> MRVKTIMTQNPVTITLPATRNYALELFKKYKVRSF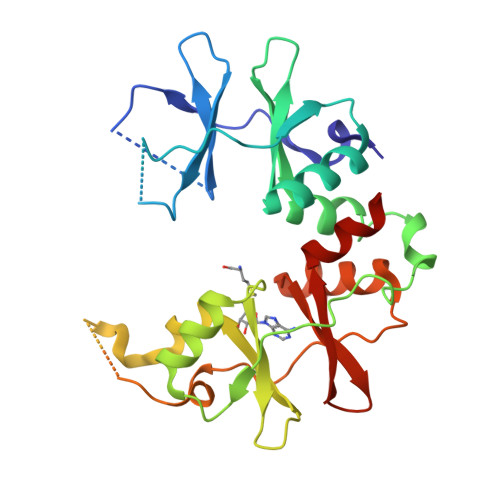PVVNKEGKLVGIISVKRILVNPDEEQLAMLVKRDVPVVKENDTLKKAAKLMLEYDYRRVVVVDSKGKPVGILTVGDIIRRYFAKSEKYKGVEIEPYYQRYVSIVWEGTPLKAALKALLLSNSMALPVVDSEGNLVGIVDETDLLRDSEIVRIMKSTELAASSEEEWILESHPTLLFEKFELQLPNKPVAEIMTRDVIVATPHMTVHEVALKMAKYSIEQLPVIRGEGDLIGLIRDFDLLKVLVKSKA> ARSTNTFNYATYHTLDEIYDFMDLLVAEHPQLVSKLQIGRSYEGRPIYVLKFSTGGSNRPAIWIDLGIHSREWITQATGVWFAKKFTEDYGQDPSFTAILDSMDIFLEIVTNPDGFAFTHSQNRLWRKTRSVTSSSLCVGVDANRNWDAGFGKAGASSSPCSETYHGKYANSEVEVKSIVDFVKDHGNFKAFLSIHSYSQLLLYPYGYTTQSIPDKTELNQVAKSAVAALKSLYGTSYKYGSIITTIYQASGGSIDWSYNQGIKYSFTFELRDTGRYGFLLPASQIIPTAQETWLGVL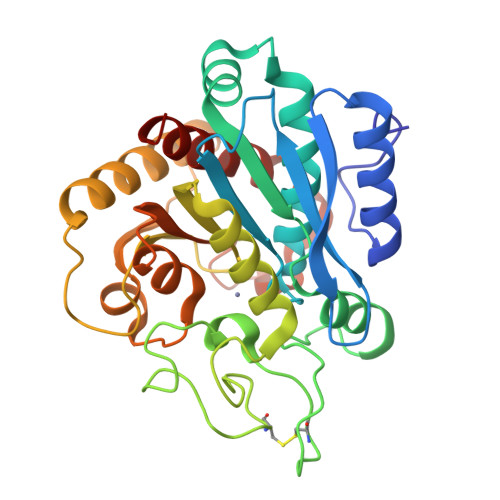TIMEHTVNNLY>[4x]MLWWEEVEDSYEREDVQKKTFTKWVNAQFSKFGKQHIENLFSDLQDGRRLLDLLEGLTGQKLPKEKGSTRVHALNNVNKALRVLQNNNVDLVNIGSTDIV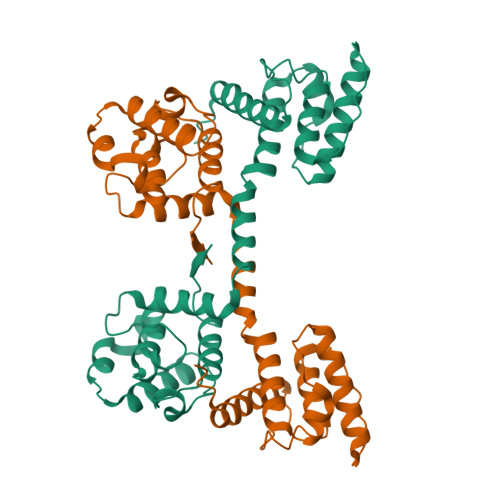DGNHKLTLGLIWNIILHWQVKNVMKNIMAGLQQTNSEKILLSWVRQSTRNYPQVNVINFTTSWSDGLALNALIHSHRPDLFDWNSVVSQQSATQRLEHAFNIARYQLGIEKLLDPEDVDTTYPDKKSILMYITSLFQVLPQQVSIE> MELFDENYYAKAVANIIGEVKDPIMYKWFSPDQIEDVDLQMGYQKTVKWDAFLNANPTTIANEVNTISTIGFSSEVVRLNYLKLQYKFRHLKQTSEKFYTSDSYIGDINNNLLPFAQAYKLASSEIIKLINHFVLTGTVSIQKDGK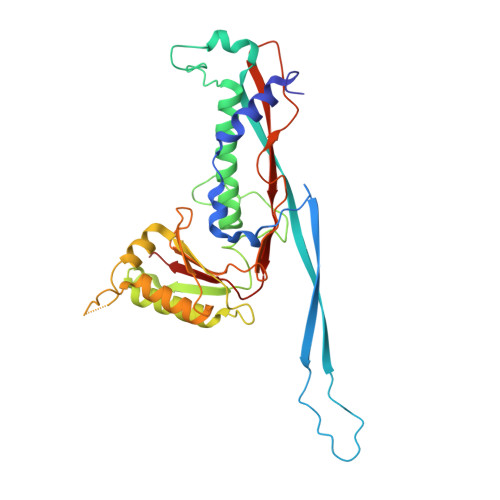NQKRLLPNMYGLLNMPEQIKEEVASGDKDKMDKIFEKIEAGLSKLELGDEFSTPMMVIVDPATSLKLVKPYAAAQGAASSCEKWEDVLIQTIKAINNREDVYIETSNLLKHKILIYPLNSELIKFKPSKYMLPTPNEQVDKDSTDVAHSYIDFVLGGLLATRKTILQVNIKQS4-{[(Z)-(7-oxo-6,7-dihydro-8H-[1,3]thiazolo[5,4-e]indol-8-ylidene)methyl]amino}benzene-1-sulfonamide | C16 H12 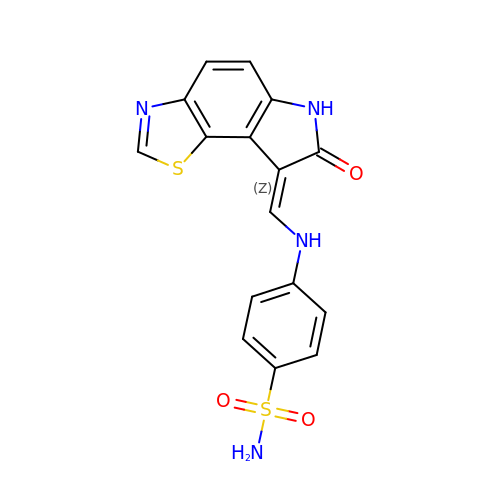N4 O3 S2 | LTYGAJVXAFJKSY-XFFZJAGNSA-N>[4x]PPHWGYFGEEGPQYWGELAPEFSTCKTGKNQSPIN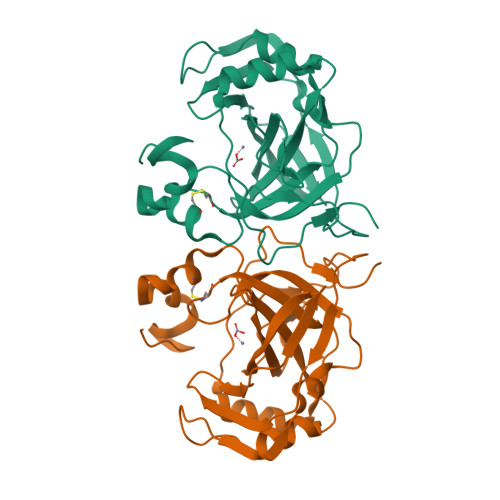LKPQTAVGTTSLPGFDVYYRETALKLINNGHTLQVNIPLGSYIKINGHRYELLQYHFHTPSEHQRDGFNYPMEMHLVHKDGDGNLAVIAILFQEGEENETLAKLMSFLPQTLKKQEIHESVKIHPAKFFPADKKFYKYSGSLTTPPCSEGVYWMVFKQPIQASVTQLEKMHEYLGSNARPVQRQNARTLLKSWPDRNA In this study we identified AFF4, a scaffold protein of the Super Elongation Complex (SEC), as an important transcriptional elongation factor required for ESR1 gene expression. In mammalian cells, the active form of P-TEFb is tightly associated with additional elongation factors ELL1/2/3, EAF1/2, AF9/ENL, as well as AFF4/1 to form the Super Elongation Complex (SEC). Importantly, AFF4, the scaffold subunit of the SEC, is largely responsible for this histone mark recognition activity. AFF4 belongs to the AFF(AF4/FMR2) family which contains four members: AFF1/AF4, AFF2/FMR2, AFF3/LAF4, and AFF4/AF5q31.

To gain a better understanding of the molecular basis by which AFF4 interacts with H3K27ac, we set out to determine the crystal structure of the C-terminal domain of AFF4. However, we did succeed in crystallizing and solving the structure of an AFF4 fragment encompassing residues 900–1163. Surprisingly, the 2.2 Å structure shows an all α-helical homodimeric structure, instead of the predominantly β-sheet YEATS domain-like structure. The ordered portion of the structure, containing residues 902–1160, with the exception of a disordered internal segment from residue 1047 to residue 1080, forms eight α-helices. Helices α5 and α6 are extensively involved in homodimerization. Phe1103, the residue identified to be important for H3K27ac interaction, is located in the middle of α6 and involved in dimerization via stacking with the same residue from another molecule. In consistent with the structural result, AFF4 dimerization was abolished by a rather large deletion of residues 971–1117, but was not affected by the single mutation F1103A in cells. Our structural result contrasts the expectation of a YEATS domain suggested by sequence alignment, and precludes direct participation of Phe1103 in H3K27ac interaction in the present form. 901–1163 domain we crystallized is not competent for H3K27ac binding in our pull-down experiment. Our structural result reveals that the 901–1163 region of AFF4 is a dimerization module, instead of a complete H3K27ac-interacting domain.

> GSKPRRTKLVFDDRNYSADHYLQEAKKLKHNADALSDRFEKAVYYLDAVVSFIECGNALEKNAQESKSPFPMYSETVDLIKYTMKLKNYLAPDATAADKRLTVLCLRCESLLYLRLFKLKKENALKYSKTLTEHLKNSYNNSQAPSPGLGSKAVGMPSPVSPKLSPGNSGNYSSGASSASASGSSVTIPQKIHQMAASYVQVTSNFLYATEIWDQAEQLSKEQKEFFAELDKVMGPLIFNASIMTDLVRYTRQGLHWLRQDAKLIS>MPLDAG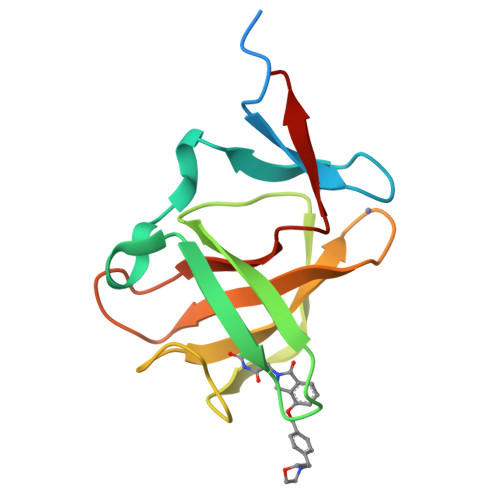GQNSTQMVLAPGASIFRCRQCGQTISRRDWLLPMGGDHEHVVFNPAGMIFRVWCFSLAQGLRLIGAPSGEFSWFKGYDWTIALCGQCGSHLGWHYEGGSQPQTFFGLIKDRLAEGPAD[3x]5-chloro-N~2~-{4-[4-(dimethylamino)piperidin-1-yl]-2-methoxyphenyl}-N~4~-[2-(dimethylphosphoryl)phenyl]pyrimidine-2,4-diamine 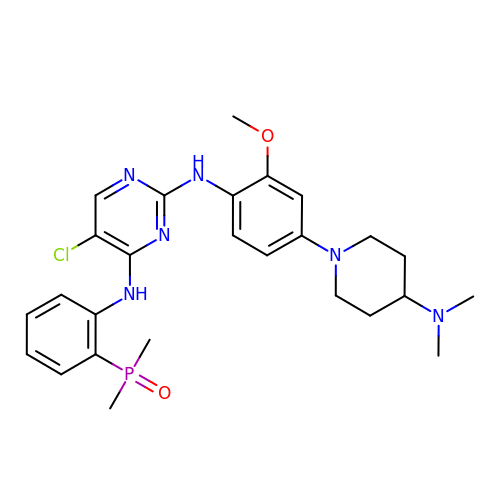| C26 H34 Cl N6 O2 P | OVDSPTSBIQCAIN-UHFFFAOYSA-N> 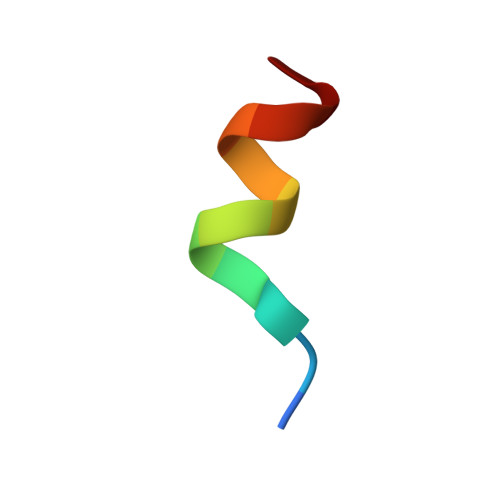RPASELLKYLTT>SHKEFTKFCYEVYNEIKISDKEFKEKRAALDTLRLCLKRISPDAELVAFGSLESGLALKNSDMDLCVLMDSRVQSDTIALQFYEELIAEGFEGAFLQAARIPIIKLTSDTKNGFGASFQCDIGFNNRLAIHNTLLLSSYTKLDARLKPMVLLVKHWAKRKQINSPYFGTLSSYGYVLMVLYYLIHVIKPPVFPNLLLSPLKQEKIVDGFDVGFDDKLEDIPPSQNYSSLGSLLHGFFAFYAYAFE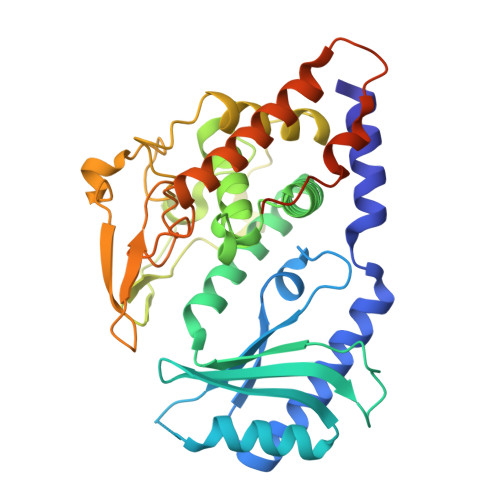PREKVVTFRRPDGYLTKQEKGWTSATEHTGSADQIIKDRYILAIEDPFEISHNVGRTVSSSGLYRIRGEFMAASRLLNSRSYPIPYDSLFEEAPIPPRRQKKTDEQSNKKLLNETDGDNSE[2x]> MRILAID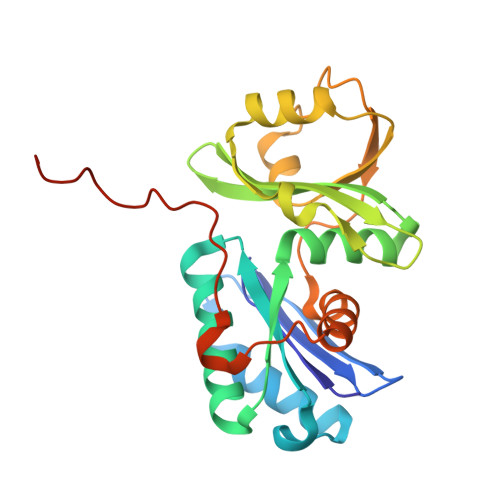TATEACSVALWNDGTVNAHFELCPREHTQRILPMVQDILTTSGTSLTDINALAYGRGPGSFTGVRIGIGIAQGLALGAELPMIGVSTLMTMAQGAWRKNGATRVLAAIDARMGEVYWAEYQRDENGIWHGEETEAVLKPEIVHERMQQLSGEWVTVGTGWQAWPDLGKESGLVLRDGEVLLPAAEDMLPIACQMFAEGKTVAVEHAEPVYLRNNVAWKKLPGKEHHHHHH> 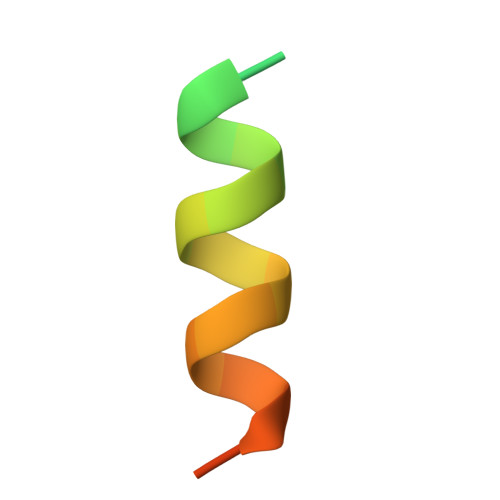NMKAGATSEGVLANFFNSLLSKKTG>[6x]SRPHQWQTDEEGVRTGKCSFPVKYLGHVEVDESRGMHICEDAVKRLKAERKFFK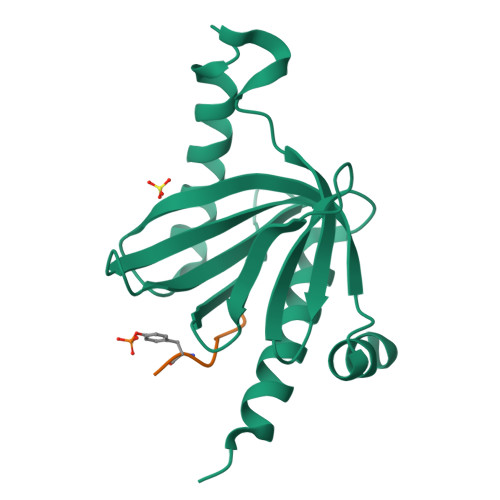GFFGKTGKKAVKAVLWVSADGLRVVDEKTKDLIVDQTIEKVSFCAPDRNFDRAFSYICRDGTTRRWICHCFMAVKDTGERLSHAVGCAFAACLERKQKREKE;>[6x]AYIGPYL> MAHHHHHHMKDNITIHPHTAGTPIPYDLLLLADPSKELIDQYLTSGELYLAKYNNEIIGCYVLYPWDFETTEIKNIAVAEKFQNQGIGGQLLKDVILKAKNKFYKKLVIGTGNSSTGQLYLYQ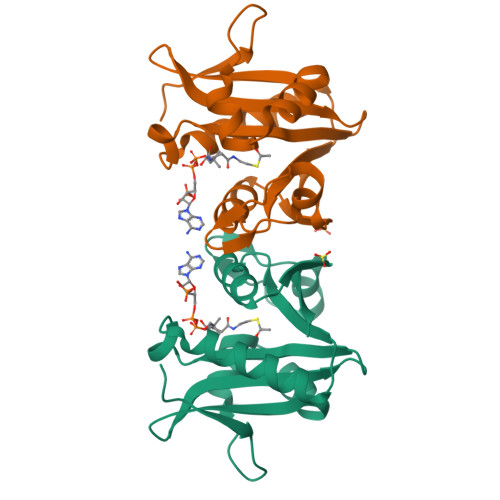KYGFRITDIRKNFFKDNYPEPIWENGIECTDMILLTMEL> GSHMEAVQ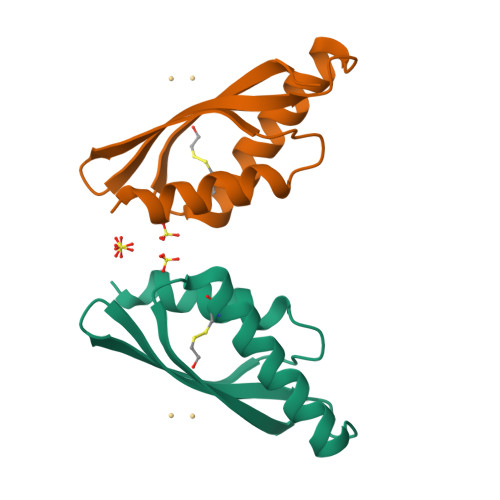NRIVEAAERVPGVRGVIHLRARYVGQDIWADMIIGVDPENTVEQAHEICEAVQAAVCGKIRRIESLHVSAEAREIGDTTKPSFSDQPLSFDEVMLSKVDN>[2x]MGKVEFSGKRYVIDGEPVTIAGGTLQFFRVPADAWKDRLLKMREAGLNTVDTYVAWNWHEPEKGSFDFKGETHPQRNLVGFLELADELGFYVIIRPGPYICGEWRNGGIPDWLIDEHPEILAKGPNGPLPRDIYYPPITYLHPTYLEAVGEWYNAVFPVIRKYLYTNGGPIISVSIDDEPSYWETIFQPFLTDYNEIITKPGGLWEKWLEQNYTLEDLRRRYKGDFKDYSEIKVPTSFSEPLPKLIDWHHFKLWMINEYVRWIYERMAREFD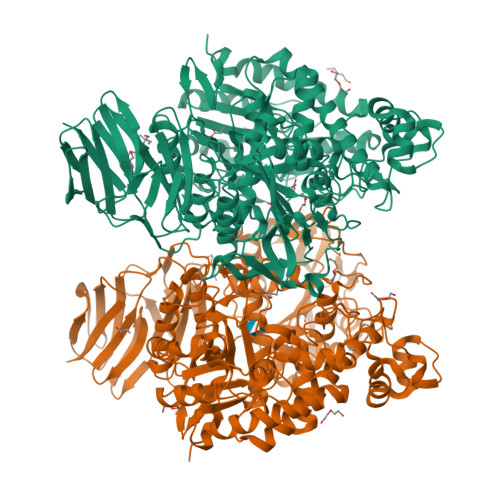VPISILDPYLLQVAWRHFFTYMREHNLKIHVWTEFWYSFYRSSDFKEDKLGHIYYKTGIYRYHVRKAGTPPLSIETQSSLAHTIDPTEAELLYSILPPLGIPNINYYLFVGGENPEGYESHNGITWDVYSPVGLDGSERPHFGVIKALSETMTSAEGLADAELRPKVAVGLYEPYEALNLWGYEGLEESTDLNEYLLGERGLFTLLAMSNTPFDAVDLEDVTLDELLSYDQLWVYSLDFMSREVQDKLVEFVARGGNLVILPMLPRYDENLEPYSSLKDFLGVEVEREKARRNPRLIQFLSVSAEGIDRMLVRNTVRGVRGGEPIAFLGEKPVGAFVRKGGGSAVVLGFRLQYYTSHHDLHRKFVWKLKELQGVREDFEVTNPDMIVLPMEGKGYAYLAVTNPRGHPIKGRISYRGLEVPVLLDGIELKRRGTLYLPFGVRKGDVEVAYATATLVMWEGDVLTFRNHLSGHSEIALKGVESVKVSGGKIVDGSDGEVLRIVIEHPGEYFEVELL>MIEIESLSRKWKNFSLDNLSLKVESGEYFVILGPTGAGKTLFLELIAGFHVPDSGRILLDGKDVTDLSPEKHDIAFVYQNYSLFPHMNVKKNLEFGMRMKKIKDPKRVLDTARDLKIEHLLDRNPLTLSGGEQQRVALARALVTNPKILLLDEPLSALDPRTQENAREMLSVLHKKNKLTVLHITHDQTEARIMADRIAVVMDGKLIQVGKPEEIFEKPVEGRVASFVGFENVLKGRVISAEQGLLRIRVGEVVIDAAGDMEVGDQVYAFLRPENIALSKSSTQSSIRNSLQGRVTEAWVLGALVRVKVDCGVPLNVLITRRSAEEMELSPGVQIYARFKASSVHVLR[2x];>MGHHHHHHHHHHSSGENLYFQGHMKAKNRKTRKFEPLTFVFSFLLLVLFLFIFLTLSNMIFEQITEDFSGLVKAAGNRSVISSIFLSLYAGFLATLLALLLGAPTGYILARFDFPGKRLVESIIDVPVVVPHTVAGIALLTVFGSRGLIGEPLESYIQFRDALPGIVVAMLF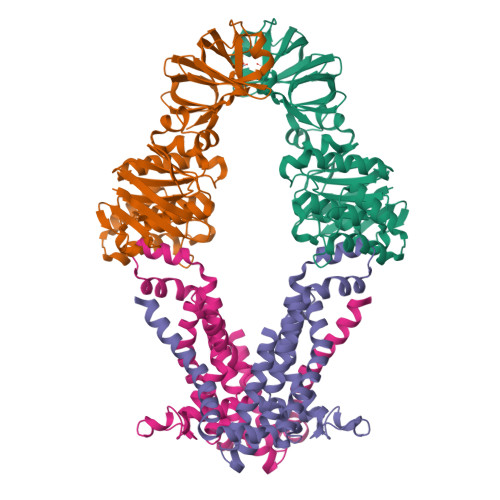VSMPYLANSAREGFKSVDPRLENAARSLGAPLWKAFFFVTLPLSARYLLIGSVMTWARAISEFGAVVILAYYPMVGPTLIYDRFISYGLSASRPIAVLLILVTLSIFLVIRTLSAGWSIYDRD[2x]5-bromouridine 5'-(tetrahydrogen triphosphate) | C9 H14 Br N2 O15 P3 | 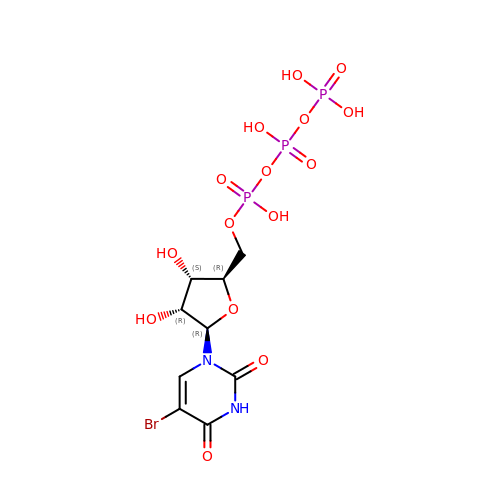IWFHOSULCAJGRM-UAKXSSHOSA-N> GSHESYTLTPEVGELIEKVRKAHQETF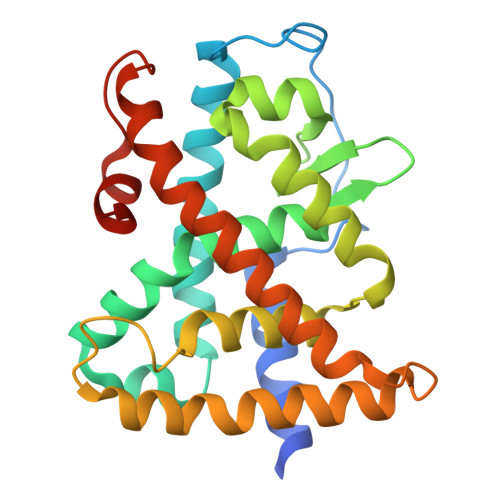PALCQLGKYTTNNSSEQRVSLDIDLWDKFSELSTKCIIKTVEFAKQLPGFTTLTIADQITLLKAACLDILILRICTRYTPEQDTMTFSDGLTLNRTQMHNAGFGPLTDLVFAFANQLLPLEMDDAETGLLSAICLICGDRQDLEQPDRVDMLQEPLLEALKVYVRKRRPSRPHMFPKMLMKITDLRSISAKGAERVITLKMEIPGSMPPLIQEMLENSEGLD> MITMKCRKCGKPSIYHQKHSGNNYCKECFIKETKRKVRKTLGRDVLKNNIKVAMGLSGGKDSLVMAYLLNEYYKQIPNSNLIAIMVNEGIEGYRTDGIDAAVKFCEEYGIEYKIVHFKDYLGTNLDEIVKIAKEKNLTMNP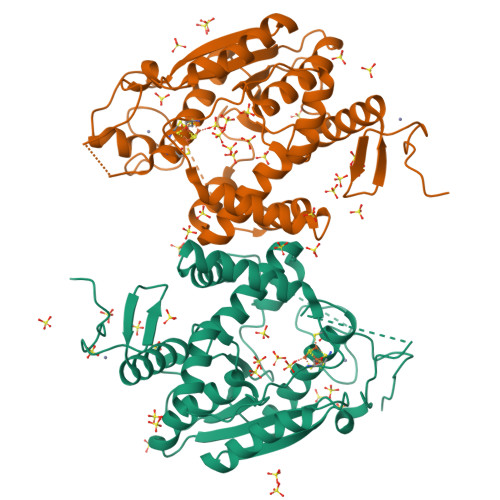CSFCGVIRRKILNRVSIEEKCDFLAIGHNLDDVAQAVMMNYIEGDVKKLAFLGKSLKHPKFVKRIKPLEKIPEDEVLLLAEMLELKYHKSPCPYSCLSFRSEVSDITDNLEKNHPGSKYSIVRGYERLLEHIELPGYTGECKICGDLSATEVCKVCSYLKNLGILEK;> MITMKCRKCGKPSIYHQKHSGNNYCKECFIKETKRKVRKTLGRDVLKNNIKVAMGLSGGKDSLVMAYLLNEYYKQIPNSNLIAIMVNEGIEGYRTDGIDAAVKFCEEYGIEYKIVHFKDYLGTNLDEIVKIAKEKNLTMNPCSFCGVIRRKILNRVSIEEKCDFLAIGHNLDDVAQAVMMNYIEGDVKKLAFLGKSLKHPKFVKRIKPLEKIPEDEVLLLAEMLELKYHKSPCPYSCLSFRSEVSDITDNLEKNHPGSKYSIVRGYERLLEHIELPGYTGECKICGGLSATEVCKVCSYGKNLGILEKSKF(2,5-dimethylphenyl) 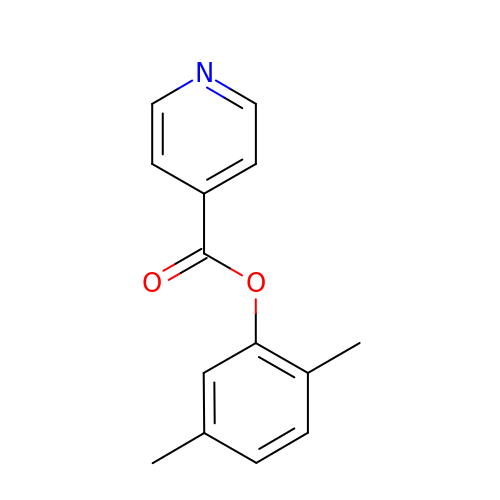pyridine-4-carboxylate | C14 H13 N O2 | MMVMRVVLUMIUAF-UHFFFAOYSA-N> SSSNSEKEWHIVPVSKDYFSIPNDLLW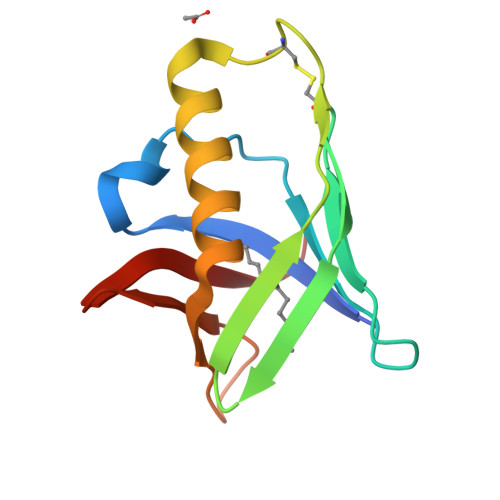SFNTTNKSINVYSKCISGKAVYSFNAGKFMGNFNVKEVDGCFMDAQKIAIDKLFSMLKDGVVLKGNKINDTILIEKDGEVKLKLIRGI>MNLVLMGLPGAGKGTQGERIVEDYGIPHISTGDMFRAAMKEETPLGLEAKSYIDKGELVPDEVTIGIVKERLGKDDCERGFLLDGFPRTVAQAEALEEILEEYGKPIDYVINIEVDKDVLMERLTGRRICSVCGTTYHLVFNPPKTPGICDKDGGELYQRADDNEE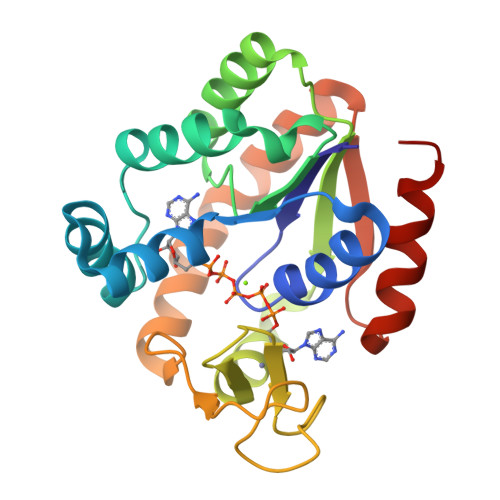TVSKRLEVNMKQIQPLLDFYSEKGYLANVNGQRDIQDVYADVKDLLGGLKK[2x]>MRGSHHHHHHGSELPQMVQQLNSPDQQELQSALRKLSQIASGGNEQIQKLIEAGALSPLVKLLDDASEEVIKNAVAAIANIAAGNNEQIQKLIEAGALSPLVKLLDDASEEVIKNAVAAIANIAAGNNEQIQKLIEAGALSPLVKLLDDASEEVIKNAVAAIANIAAGNNEQIQKLIEAGALSPLVKLLDDASEEV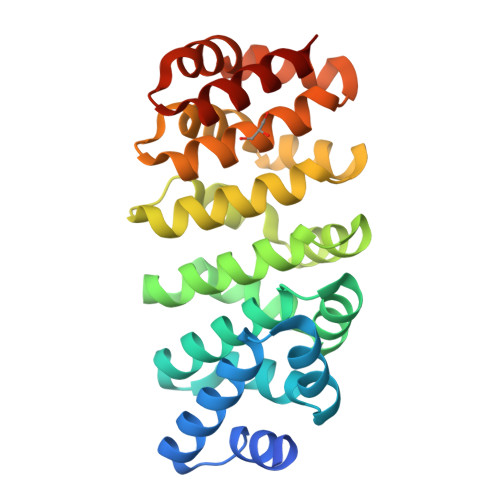IKNAVAAIANIAAGNNEMKQKLEEAGALPALEKLQSHANEEVQKNAQAALEAFNS[2x]> MADHSASGAPALSTNIESGKFDEKAAEAAAYQPKPKVEDDEDEDIDALIEDLESHDGHDAEEEEEEATPGGGRVVPEDMLQ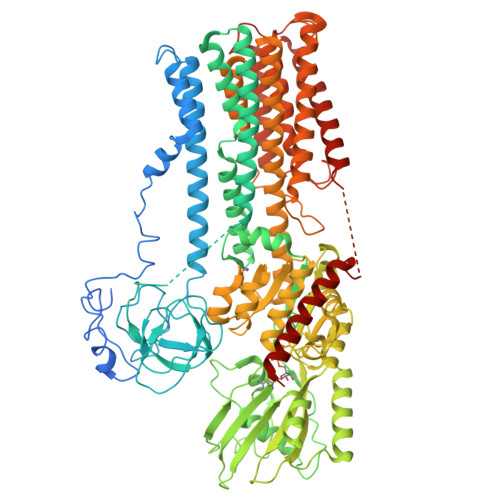TDTRVGLTSEEVVQRRRKYGLNQMKEEKENHFLKFLGFFVGPIQFVMEGAAVLAAGLEDWVDFGVICGLLLLNAVVGFVQEFQAGSIVDELKKTLALKAVVLRDGTLKEIEAPEVVPGDILQVEEGTIIPADGRIVTDDAFLQVDQSALTGESLAVDKHKGDQVFASSAVKRGEAFVVITATGDNTFVGRAAALVNAASGGSGHFTEVLNGIGTILLILVIFTLLIVWVSSFYRSNPIVQILEFTLAITIIGVPVGLPAVVTTTMAVGAAYLAKKKAIVQKLSAIESLAGVEILCSDKTGTLTKNKLSLHDPYTVAGVDPEDLMLTACLAASRKKKGIDAIDKAFLKSLKYYPRAKSVLSKYKVLQFHPFDPVSKKVVAVVESPQGERITCVKGAPLFVLKTVEEDHPIPEEVDQAYKNKVAEFATRGFRSLGVARKRGEGSWEILGIMPCMDPPRHDTYKTVCEAKTLGLSIKMLTGDAVGIARETSRQLGLGTNIYNAERLGLGGGGDMPGSEVYDFVEAADGFAEVFPQHKYNVVEILQQRGYLVAMTGDGVNDAPSLKKADTGIAVEGSSDAARSAADIVFLAPGLGAIIDALKTSRQIFHRMYAYVVYRIALSIHLEIFLGLWIAILNRSLNIELVVFIAIFADVATLAIAYDNAPYSQTPVKWNLPKLWGMSVLLGVVLAVGTWITVTTMYAQGENGGIVQNFGNMDEVLFLQISLTENWLIFITRANGPFWSSIPSWQLSGAIFLVDILATCFTIWGWFEHSDTSIVAVVRIWIFSFGIFCIMGGVYYILQDSVGFDNLMHGKSPKGNQKQRSLEDFVVSLQRVSTQHEKSQ> GSHMAAVDLATHPGHLARRLQQAHYLLWNTMVSEETTSPQYAVLNALVAEPGLDQRTVGERVGLDRSTIAEVVSRLGRRGLLDKVRDPQDG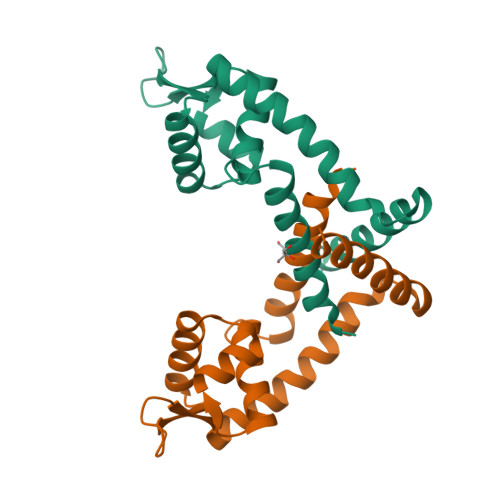RRSLLRLTDEGLRVHRRLGVRIARMNQVFLAPLAADEQAVFFDLIRRVADAAEGLRNPAEPAVAPG>MISKRLELVASFVSQGAILLDVGSDHAYLPIELVERGQIKSAIAGEVVEGPYQSAVKNVEAHGLKEKIQVRLANGLAAFEETDQVSVITIAGMGGRLIARILEEGLGKLANVERLILQPNNREDDLRIWLQDHGFQIVAESILEEAGKFYEILVVEAGQMKLSASDVRFGPFLSKEVSPVFVQKWQKEAEKLEFALGQIPEK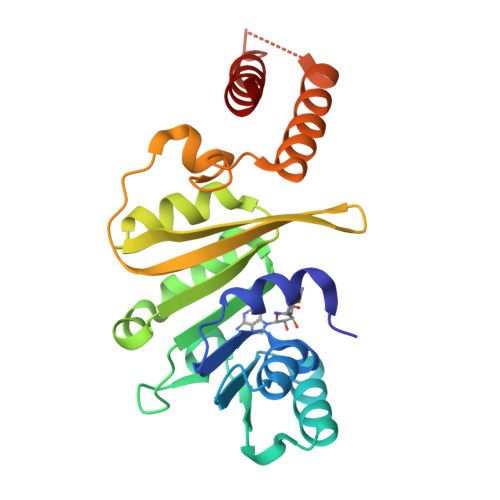NLEERQVLVDKIQAIKEVLHVSK[8x]> GSSAVNQENERLMEEYERLASELLEWIRRTIPWLENRTPEKTMQAMQKKLEDFRDYRRKHKPPKVQEKCQLEINFNTLQTKLRISNRPAFMPSEGKMVSDIAGAWQRLEQAEKGYEEWLLNEIRRLERLEHLAEKFRQKASTHETWAYGKEQILLQKDYESASLTEVRALLRKHEAFESDLAAHQDRVEQIAAIAQELNELDYHDAVNVNDRCQKICDQWDRLGTLTQKRREALERMEKLLETIDQLHLEFAKRAAPFNNWME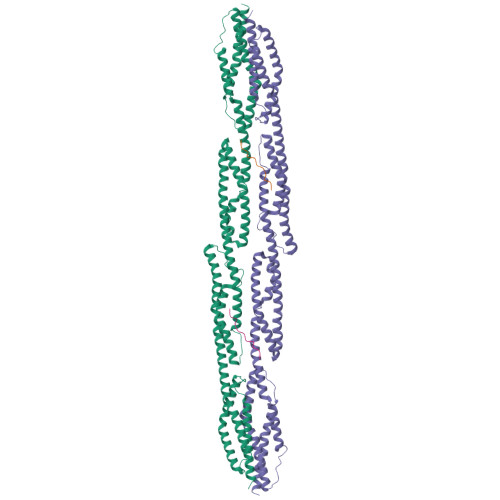GAMEDLQDMFIVHSIEEIQSLITAHEQFKATLPEADGERQSIMAIQNEVEKVIQSYNIRISSSNPYSTVTMDELRTKWDKVKQLVPIRDQSLQEELARQHANERLRRQFAAQANAIGPWIQNKMEEIARSSIQITGALEDQMNQLKQYEHNIINYKNNIDKLEGDHQLIQEALVFDNKHTNYTMEHIRVGWELLLTTIARTINEVETQILTRD;> GPTVGGQLGTAGQGFSYSKSNGRGGSQAGGSGSAGQYGSDQQHHLGSGSGAGGTGGPAGQAGRGGAAGTAGVGETGSGDQAGGEGKHITVFKTYISPWERAMGVDPQQKMELGIDLLAYGAKAELPKYKSFNRTAMPYGGYEKASKRMTFQMPKFDLGPLLSEPLVLYNQNLSNRPSFNRTPIPWLSSGEPVDYNVDIGIPLDGETEEL~{tert}-butyl 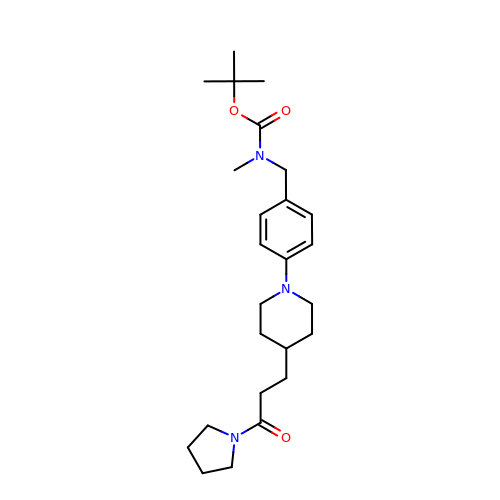~{N}-methyl-~{N}-[[4-[4-(3-oxidanylidene-3-pyrrolidin-1-yl-propyl)piperidin-1-yl]phenyl]methyl]carbamate | C25 H39 N3 O3 | IWVJBZLBIWIKGF-UHFFFAOYSA-N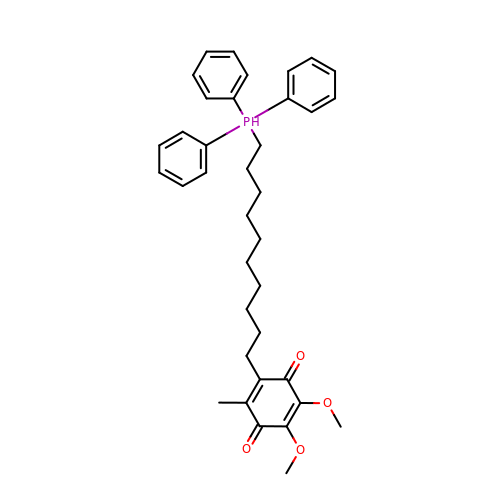2,3-dimethoxy-5-methyl-6-[10-(triphenyl-$l^{5}-phosphanyl)decyl]cyclohexa-2,5-diene-1,4-dione | C37 H45 O4 P | BIPKQWZPPRRUAP-UHFFFAOYSA-N> MATQFKMDSVPGSLVVVGGTYEPWLSVLEQVGWKCHQCADLRKVDALLEDIGPCIGIVDLSHDEFSLNGIANLVSTHKHVRWLAFIREQQLSSDTICQFIVNFCIDFFT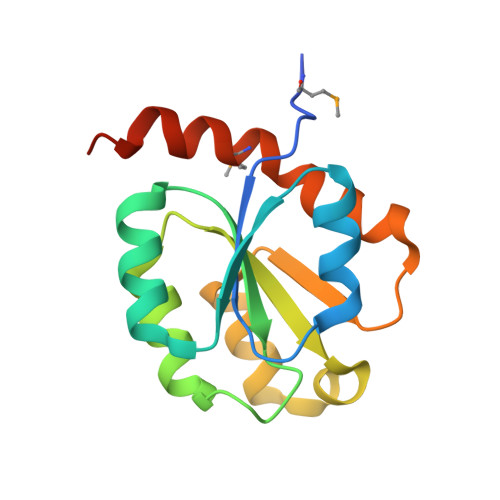APIPDAQLLSTIGHQLGMLKLEKKVWPTFGNNQDM> SNAGVSDVELRVALPDGTTVTVRVKKNSTTDQVYQAIAAKVGMDSTTVNYFALFEVISHSFVRKLAPNEFPHKLYIQNYTSAVPGTCLTIRKWLFTTEEEILLNDNDLAVTYFFHQAVDDVKKGYIKAEEKSYQLQKLYEQRKMVMYLNMLRTCEGYNEIIFPHCACDSRRKGHVITAISITHFKLHACTEEGQLENQVIAFEWDEMQRWDTDEEGMAFCFEYARGEKKPRWVKI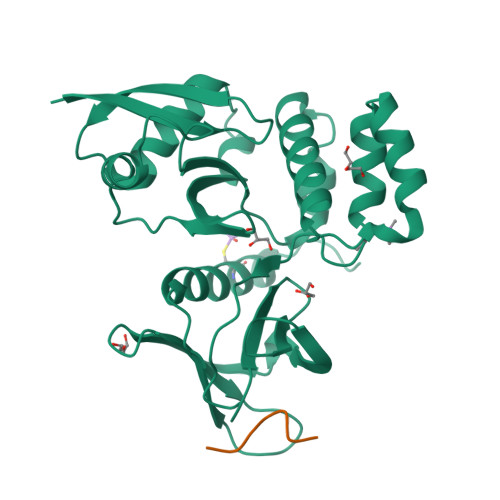FTPYFNYMHECFERVFCELKWRKEEY;> NLFDDNIDIFADLT> M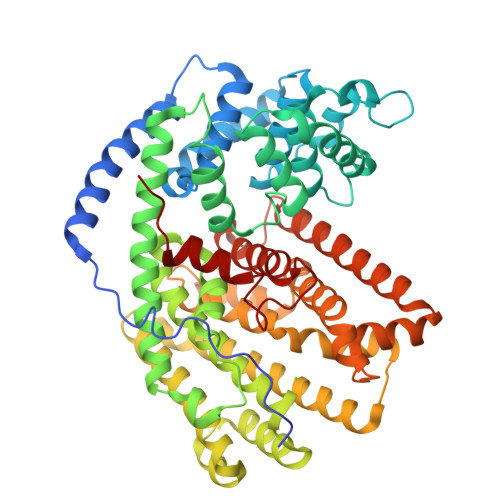ASAAVANYEEEIVRPVADFSPSLWGDQFLSFSIDNQVAEKYAKEIEALKEQTRNMLLATGMKLADTLNLIDTIERLGISYHFEKEIDDILDQIYNQNSNCNDLCTSALQFRLLRQHGFNISPEIFSKFQDENGKFKESLASDVLGLLNLYEASHVRTHADDILEDALAFSTIHLESAAPHLKSPLREQVTHALEQCLHKGVPRVETRFFISSIYDKEQSKNNVLLRFAKLDFNLLQMLHKQELAQVSRWWKDLDFVTTLPYARDRVVECYFSALGVYFEPQYSQARVMLVKTISMISIVDDTFDAYGTVKELEAYTDAIQRWDINEIDRLPDYMKISYKAILDLYKDYEKELSSAGRSHIVCHAIERMKEVVRNYNVESTWFIEGYTPPVSEYLSNALATTTYYYLATTSYLGMKSATEQDFEWLSKNPKILEASVIIWRVIDDTATYEVEKSRGQIATGIECCMRDYGISTKEAMAKFQNMAETAWKDINEGLLRPTPVSTEFLTPILNLARIVEVTYIHNLDGYTHPEEVLKPHIINLLVDSIKI(1R,4R)-4-fluoro-3-[({3-hydroxy-2-methyl-5-[(phosphonooxy)methyl]pyridin-4-yl}methyl)amino]cyclopent-2-ene-1-carboxylic acid | 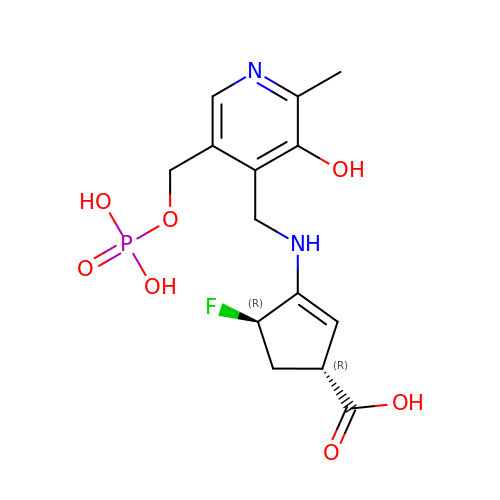C14 H18 F N2 O7 P | YUSFTNIOKSVGAN-LDYMZIIASA-N>MNEAGQKKTDKDRVLSLDAATIVGEQQDETTYNVDRSASKKYTAPLLDTPKTVTVIPQQVIKDTGALTLADALRTTPGITFGAGEGGNPAGDRPFIRGFNAESDTFLDGMRDVASQTREVFNVEQIEVSKGPGSAYTGAGSTGGSLNLISKTAKQDNFTDAGFTWGSDQTRRTTLDVNRMIGDNAAFRLNLMKHDAHVAGRDEVSVSRWGVAPTVTFGFDTPTRATLSYYHLSTDDMPDYGLPLTNVNRSKANPSKPASVDRDNFYGLKDRDYRKSTTDSGTFRIEHDLNDNLTLSNSTRLVRTTLDYIVSNPDDSRGNVANGYVYRSAKSRNSTSKGWVNQTDLKANFETGFIKHTLVTGLEFSYEDVHNRPYAITSGGGAGNTCNARLLASGDCTSLNRPTPGDNWTGSITDGLAYTDTDTKTSAAYVFDTLKLSEQWELNLGLRYDDFDTKSSGYQTAGRNGPAGYFKRENNSHFWNYQTGLVYKPAPNGSIYLAWSTSSNPTGETGGEGQADISVGNNGLDPERNRNLELGTKWAFFDDALSLNAALFRTDKTNARVASPDVSTLQVLDGEQRVQGVELGFNGKLTEKWKVFGGYTYLDSEIRKSTVKSDEGNKMPQTAQNNFTLWTTYDLLQNFTIGGGTTY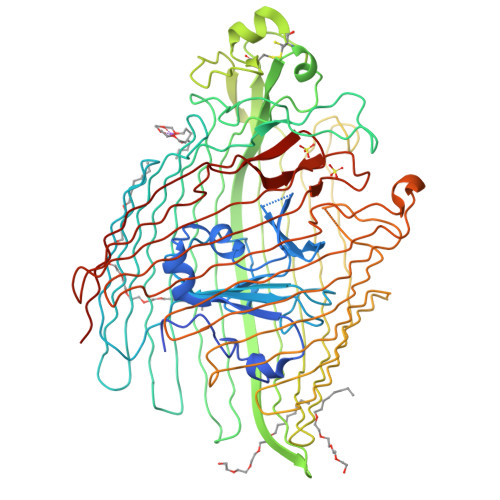VDKQYGNTANSTYIPSYWRYDAMASYKVSKNVDLQLNVQNLTDKRYFDQVYSTHMAHVAPGRTALLGVNFHFSAALEHHHHHH[2x]N-benzyl-N-(3-tert-butyl-4-hydroxyphenyl)-2,6-dichloro-4-(dimethylamino)benzamide | C26 H28 Cl2 N2 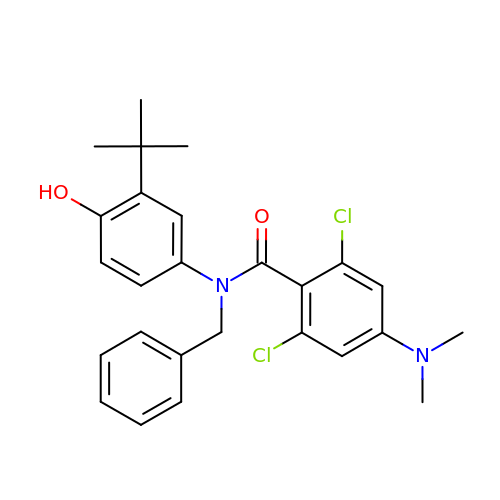O2 | IDACWMHIKWNAEO-UHFFFAOYSA-N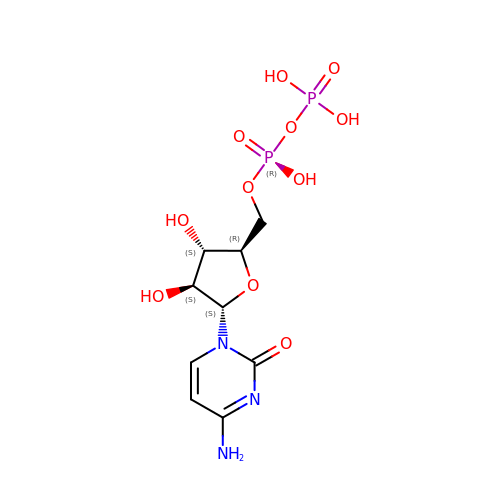4-AMINO-1-{5-O-[(R)-HYDROXY(PHOSPHONOOXY)PHOSPHORYL]-ALPHA-D-ARABINOFURANOSYL}PYRIMIDIN-2(1H)-ONE | C9 H15 N3 O11 P2 | ZWIADYZPOWUWEW-GVYWOMJSSA-N>MNKKRLLLLSVFLVSVFVPVLVADVIYYYQGQITVGNVAPPMYFAIQPNGNAKIGNNSNVPSYINAQPSSGGSGFTAQVNITNATYNYYFNFMGLAVSKTGYIYLAKVAYSYTATNNPIQNATLYIMNQQGQIVYKYKLIVNGVVNSTLPSTPLQINSGSYIVSLLIVPYQGTLPKT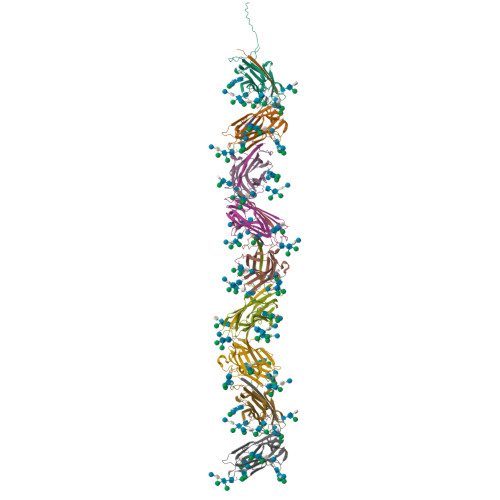PSNDLATITVNFGFSPMTASPPPIPLPSP[9x]>[2x]MGSSHHHHHHSSGR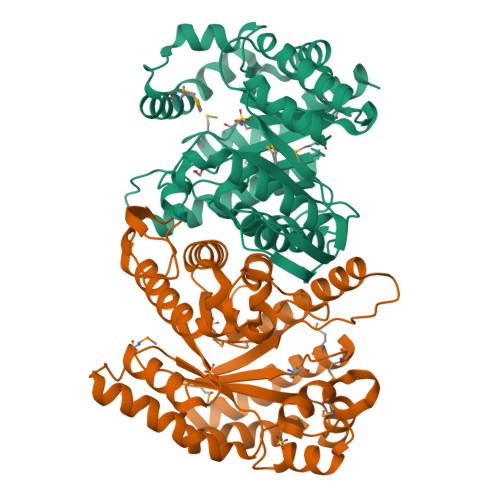ENLYFQGMELGLYTFADVNPNPADGRGPEGARRLRELLEEIELADQVGLDVFGLGEHHRPDYVVSSPSTVLAAAAVKTKNIRLTSAVSVLSSDDPVRVFQQFSTVDLLSNGRAEIMAGRGSFIESYPLFGYDLEDYDVLFAEKLDLLLALREQEVVTWSGTKHPAINGRGVYPRPLQERLPVWIAVGGTPQSVARAGAMGLPVALAIIGGEYRRFAPLFDLYHEAARRAGQEKTKLRTSINVHGFIADTTDKAADQFYGPQAEVMNRIGRERGWGPTNRAHFDAARGPEGNLFLGEPELVAEKIIKAHGVFKNDRFLLQMAIGLMPHDQIMRGIELYGTKVAPLVRKELTGSADPVKATAGS>DGRYSLTYIYTGLSKHVEDVPAFQALGSLNDLQFFRYNSKDRKSQPMGLWRQVEGMEDWKQDSQLQKAREDIFMETLKDIVEYYNDSNGSHVLQGRFGCEIENNRSSGAFWKYYYDGKDYIEFNKEIPAWVPFDPAAQITKQKWEAEPVYVQRAKAYLEEECPATLRKYLKYSKNILDRQDPPSVVVTSHQAPGEKKKLKCLAYDFYPGKIDVHWTRAGEVQ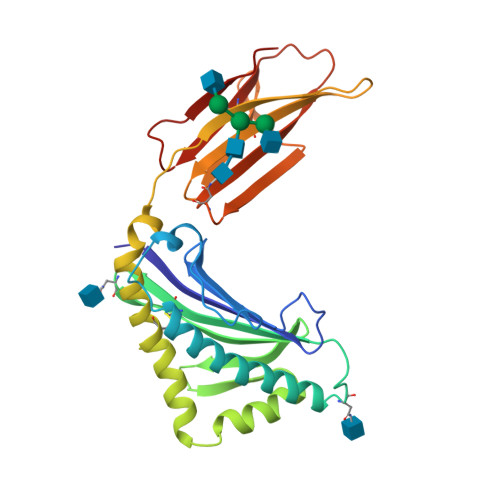EPELRGDVLHNGNGTYQSWVVVAVPPQDTAPYSCHVQHSSLAQPLVVPWEAS[4x]> EIIPRCELVKILREHGFEGFEGTTIADWIC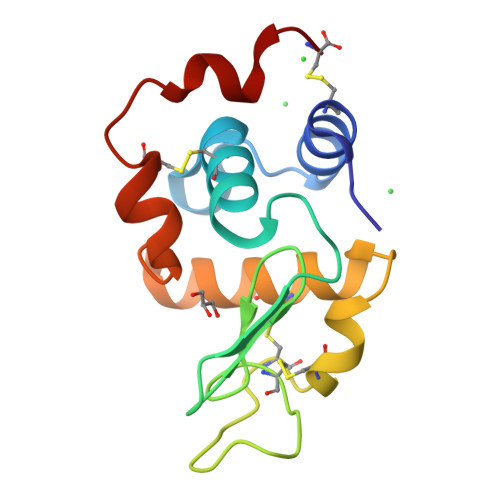LVQHESDYNTEAYNNNGPSRDYGIFQINSKYWCNDGKTSGAVDGCHISCSELMTNDLEDDIKCAKKIARDAHGLTPWYGWKNHCEGRDLSSYVKGC> MKQDASRNAAYTVDCEDYVHVVEFNPFENGDSGNLIAYGGNNYVVIGTCTFQEEEADVEGIQYKTLRTFHHGVRVDGIAWSPETRLDSLPPVIKFCTSAADMKIRLFTSDLQDKNEYKVLEGHTDFINGLVFDPKEGQEIASVSDDHTCRIWNLEGVQTAHFVLHSPGMSVCWHPEETFKLMVAEKNGTIRFYDLLAQQAILSLESEQVPLMSAHWCLKNTFKVGAVAGNDWLIWDITRSSYPQNKRPVHMDRACLFRWSTISENLFATTGYPG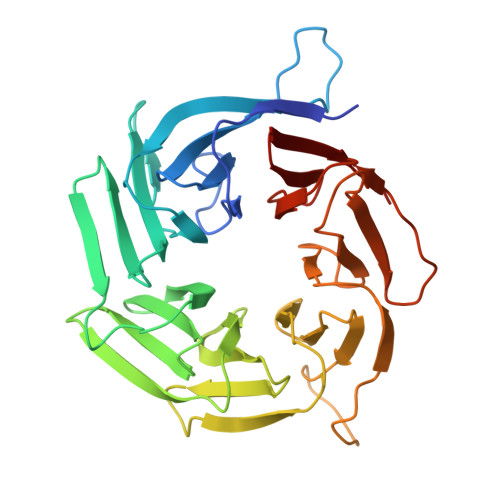KMASQFQIHHLGHPQPILMGSVAVGSGLSWHRTLPLCVIGGDHKLLFWVTEV> K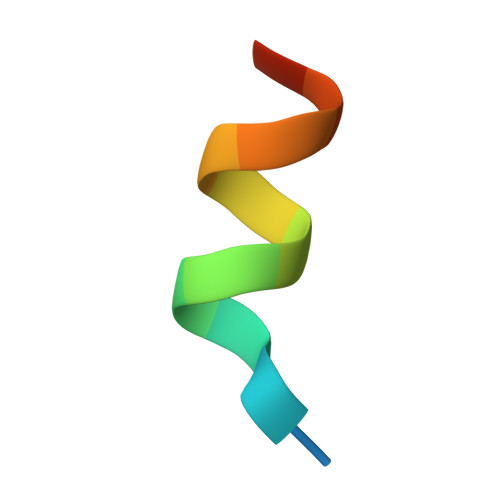DHQLLRYLLDKDE>[10x]MLVSVYLALLVACVGQAHSQANLMRLKSDLFNRSPMYPGPTKDDPLTVT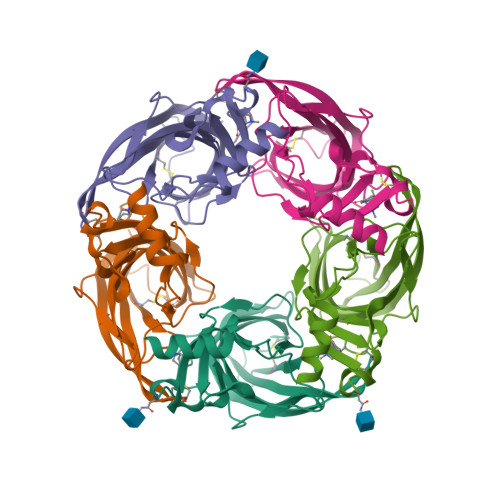LGFTLQDIVKVDSSTNEVDLVYYEQQRWKLNSLMWDPNEYGNITDFRTSAADIWTPDITAYSSTRPVQVLSPQIAVVTHDGSVMFIPAQRLSFMCDPTGVDSEEGVTCAVKFGSWVYSGFEIDLKTDTDQVDLSSYYASSKYEILSATQTRQVQHYSCCPEPYIDVNLVVKFRERRAGNGFFRNLFDENLYFQGHHHHHH9-[(2R,3R,4R)-5-(hydroxymethyl)-3-methoxy-4-oxidanyl-oxolan-2-yl]-3H-purine-2,6-dione 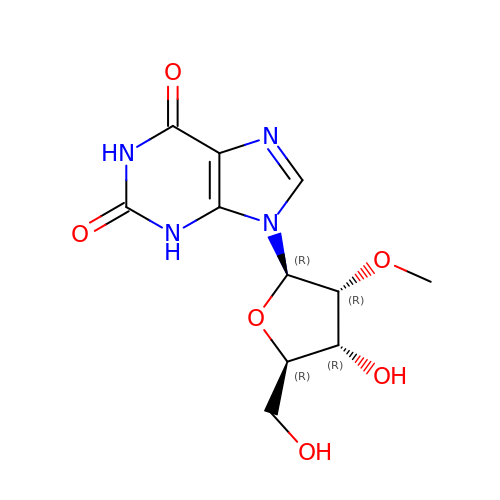| C11 H14 N4 O6 | PASFATVSJBQETG-KQYNXXCUSA-N> MDFDDDI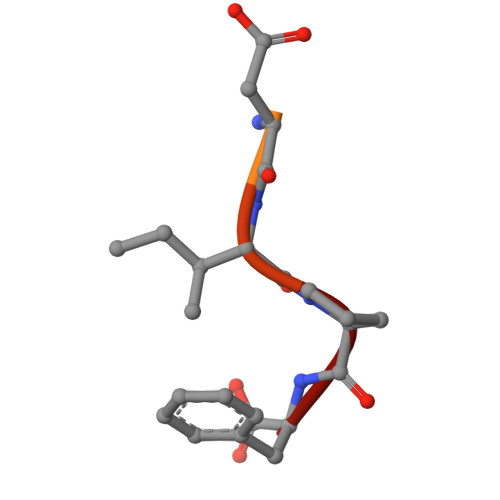PF>MAFDECACYTTRRAARQLGQAYDRALRPSGLTNTQFSTLAVISLSEGSAGIDLTMSELAARIGVERTTLTRNLEVMRRDGLVRVMAGADARCKRIELTAKGRAA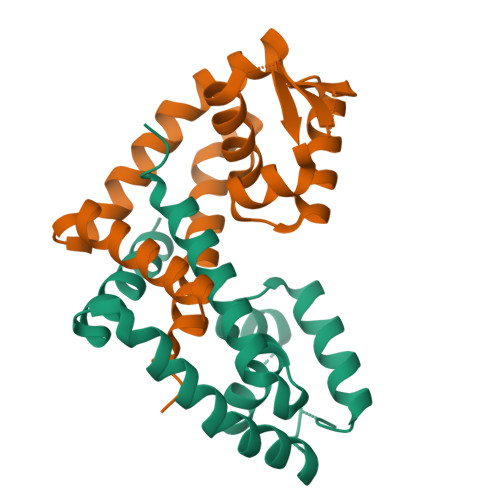LQKAVPLWRGVQAEVTASVGDWPRVRRDIANLGQAAEACRLVPR[2x]> ARECPGKQEWPELVG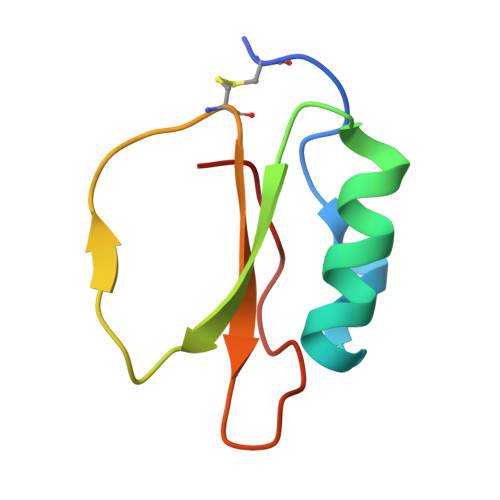EYGYKAAAIIERENPNVRSIVKHERSGFTKDFRCDRVWVVVDSTGVVVRTPRVT> MGSDKIHHHHHHENLYFQGMIIRYATPDDIEDMVSIFIDAYNFPGPRESVKSSFEISLEVQPDGCLLAFLKDEPVGMGCIFFYNKQAWIGLMGVKKAYQRRGIGTEVFRRLLEIGRRKVDTIRLDASSQGYGLYKKFKFVDEYRTVRYELMERPIKRVEGVVEVNKIPNWVKEIDKKAFGDDRIRVLEAYMRRGARLLCAENEGFGLVYRGKIGPLVADSPRVAEKILLKAFQLGAREIIIPEVNKDALELIKIFK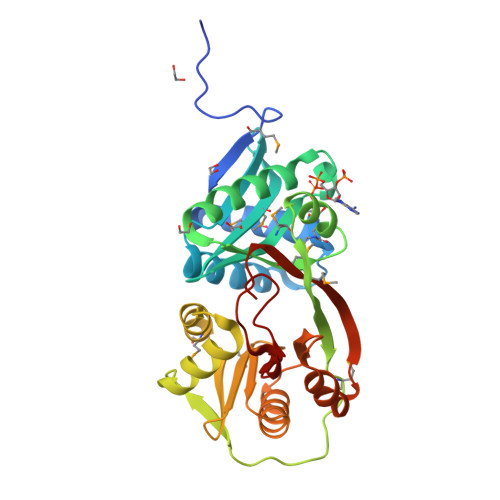PSQVTSCMRMRLGSKIEEKVDIYYGILAYAKG>MSNVQTGAERMPHDLSHLGFLAGQIGRLITISTTPVIAGDSFEMDAVGALRLSPLRRGLAIDSTVDIFTFYVPHRHVYGEQWIKFMKDGVNAAPLPTVNTTGYIDHAAFLGTINPDTNKIPKHLFQGYLNIYNNYFKAPWMPDRTEANPNQLNEDDARYGFRCCHLKNIWTAPLPPETELSRQMTTSTTSIDIMGLQAAYANLHTDQERDYFMQRYRDVISSFGGKTSYDADNRPLLVMRSNFWASGYDVDGTDQTSLGQFSGRVQQTYKHSVPRFFVPEHGTMFTLALVRFPPTATKEIQYLNAKGALTYTDIAGDPALYGNLPPREISMKDVFRSGDASKKFKIAEGQWYRYAPSYVSPAYHLLEGFPFIQEPPSGDLQERVLIRHHDYDQCFQSVQLLQWNSQVKFNVTVYRNLPTTRDSIMTS[60x];>[60x]MFQTFISRHNSNFFSDKLVATSVTPASLAPVLQTPKAASSTLYFNQLTVNAGNGGFLHCIQMDTSVNAANQVVSVGADIAFDADPKFFACLVRFESASVPTTLPTDYDVYPLDGRHDGGYYTVKDCVTIDVLPREPGNNVYVGFMVWSNFTATKCRGLVSLNQVIKEIICLQPLK;>[60x]MSKGKKRSGARPGRPQP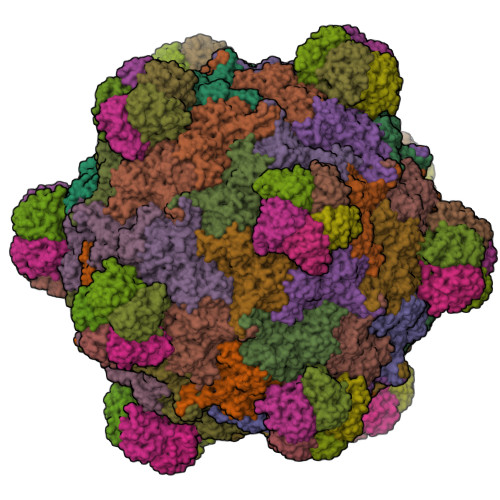LRGTKGKRKGARLWYVGGQQF>GPDYKFWYTQPVPKINDEFNESVNEPFISDNKVEDVRKDEYKLPPGYSWYVCDVKDEKDRSEIYTLLTDNYVEDDDNIFRFNYSAEFLLWALTSPNYLKTWHIGVKYDASNKLIGFISAIPTDICIHKRTIKMAEVNFLCVHKTLRSKRLAPVLIKEITRRINLENIWQAIYTAGVYLPKPVSDARYYHRSINVKKLIEIGFSSLNSRLTMSRAIKLYRVEDTLNIKNMRLMKKKDVEGVHKLLGSYLEQFNLYAVFTKEEIAHWFLPIENVIYTYVNEENGKIKDMISFYSLPSQILGNDKYSTLNAAYSFYNVTTTATFKQLMQDAILLAKRNNFDVFNALEVMQNKSVFEDLKFGEGDGSLKYYLYNWKCASFAPAHVGIVLL[3x]

N-myristoyltransferase (NMT) is a promising antimalarial drug target. NMT cotranslationally transfers the myristate moiety of myristoyl-coenzyme A (MyrCoA) to Gly2 of protein substrates after removal of the N-terminal methionine.17−19P. vivax and P. falciparum express a single NMT protein, whereas human cells express two closely related isotypes, HsNMT1 and HsNMT2.20PvNMT and PfNMT have more than 80% shared identity, while the human orthologs are only about 40% identical in sequence to PvNMT and PfNMT. Small-molecule inhibitors bind both PvNMT and HsNMT1 in the peptide binding cleft, where residues contacting the ligands via side chain atoms share 100% sequence identity. The inhibitor binding site is located within the peptide binding cleft formed by the N- and C-terminal domains.

Compound 10b adds additional volume in the core A group via the naphthalene moiety. Tyr211 adopts the selective conformation described previously. However, the bulkiness of 10b causes an additional “vertical” displacement that relieves hypothetical clashes revealed through structural superpositions. There is an accompanying rotation of Phe105. The displacement of the pyrazole group of 10b causes a more significant outward shift of the Ab loop (observed at Asp98) and weakens the hydrogen bonding with Ser319. The morpholinomethanone group anchors to Asn365 via hydrogen bonding with the ether oxygen in all asymmetric unit chains, despite conformational variability observed within the morpholine ring itself. Despite its volume, the naphthalene group does not displace the waters that extend the channel to the Tyr315 side chain and Leu409 carbonyl sites, although differences in the water structure are observed between the three chains and the occupancies differ. A second hypothesis is that the bulkiness of 10b introduces a number of additional binding site perturbations that have a compounded effect on selectivity. These include the more extensive movements observed at the inner wall (rise of Tyr211), Ab loop (outward displacement of Asp98), and “pommel horse” residue (rotation of Phe105).>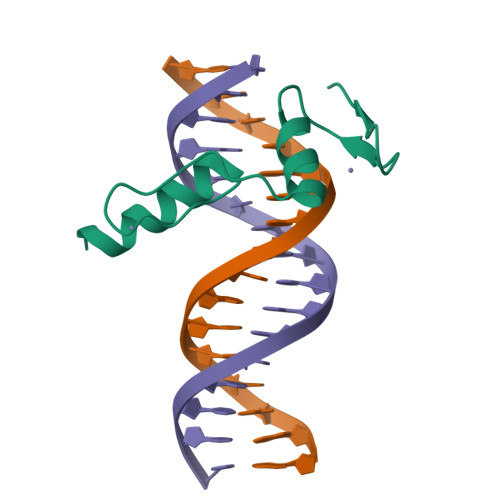GPLGSQKVEKKIRAKAFQKCPICEKVIQGAGKLPRHIRTHTGEKPYECNICKVRFTRQDKLKVHMRKHTGEKPYLCQQCGAAFAHNYDLKNHMRVHTGLRPYQCDSCCKTFVRSDHLHRHLKKDGCNGVPSRRGRKLERPHRD[3x]> GSFVEMVDNLRGKSGQGYYVEMTVGSPPQTLNILVDTGSSNFAVGAAPHPFLHRYYQRQLSSTYRDLRKGVYVPYTQGKWEGELGTDL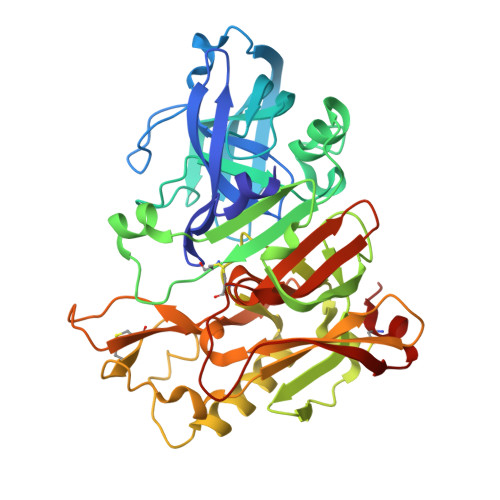VSIPHGPNVTVRANIAAITESDKFFINGSNWEGILGLAYAEIARPDDSLEPFFDSLVKQTHVPNLFSLQLCGAGFPLNQSEVLASVGGSMIIGGIDHSLYTGSLWYTPIRREWYYEVIIVRVEINGQDLKMDCKEYNYDKSIVDSGTTNLRLPKKVFEAAVKSIKAASSTEKFPDGFWLGEQLVCWQAGTTPWNIFPVISLYLMGEVTNQSFRITILPQQYLRPVEDVATSQDDCYKFAISQSSTGTVMGAVIMEGFYVVFDRARKRIGFAVSACHVHDEFRTAAVEGPFVTLDMEDCGYNI>[3x]MATKGTKRSYEQMETDGERQNATEIRASVGKMIDGIGRFYIQMCTELKLSDYEGRLIQNSLTIERMVLSAFDERRNKYLEEHPSAGKDPKKTGGPIYRRVDGKWRRELILYDKEEIRRIWRQANNGDDATAGLTHMMIWHSNLNDATYQRTRALVRTGMDPRMCSLMQGSTLPRRSGAAGAAVKGVGTMVMELIRMIKRGINDRNFWRGENGRRTRIAYERMCNILKGKFQTAAQRTMVDQVRESRNPGNAEFEDLIFLARSALILRGSVAHKSCLPACVYGSAVASGYDFEREGYSLVGIDPFRLLQNSQVYSLIRPNENPAHKSQLVWMACHSAAFEDLRVSSFIRGTKVVPRGKLSTRGVQIASNENMETMESSTLELRSRYWAIRTRSGGNTNQQRASSGQISIQPTFSVQRNLPFDRPTIMAAFTGNTEGRTSDMRTEIIRLMESARPEDVSFQGRGVFELSDEKATSPIVPSFDMSNEGSYFFGDNAEEYDN

Following increased insights into the importance of vRNPs, antiviral drugs that target nucleoprotein (NP) are an attractive strategy as NP is a highly conserved multifunctional protein that plays an essential role in infection by all subtypes of IAVs during the virus infection life cycle. NP was reported to interact with RNA and oligomerize by self-interaction to form an oligomer to maintain the structure of RNP. In addition, NP is essential for viral transcription and replication; the major role of NP is the encapsidation of RNA into an RNP complex and maintenance of the conformation of the RNA template in a suitable order for transcription, replication, and assembly into virions. Furthermore, NP or RNPs participate in translocation between the cytoplasm and nucleus with the help of other viral proteins and host factors.

Here, we characterized a novel influenza A virus nucleoprotein (NP) inhibitor, FA-6005, that inhibited a broad spectrum of human pandemic and seasonal influenza A and B viruses in vitro and protects mice against lethal influenza A virus challenge. To obtain structural insights into the interaction between NP and FA-6005, FA-6005 was cocrystallized with NP, and the complex structure was determined. The NP/FA-6005 complex crystal belongs to space group C2221, with only one NP trimer in each asymmetric unit. Three FA-6005 molecules were found in each trimer. One was in the I41 pocket, and the major interactions involved in the I41 pocket included (i) hydrophobic interactions of the t-butyl group with G288, V285, and A286, ring C with I41, and ring D with G54 and R55; (ii) hydrogen bonding between amide O2 and T45; and (iii) dipole-dipole interactions of ring D with D51 and S283. The second one was in the Y289 pocket, and the interactions involved in the Y289 pocket included hydrophobic interactions of the t-butyl group and ring A with Y289, R305, and L306 and rings A and B with N309. The third one was around N224. However, N224 might not be a real pocket since the compound is seated between two symmetry-related NP molecules. We found that in the presence of FA-6005, mutation of residues in the I41 pocket displayed high resistance, while that of residues in the Y289 pocket exhibited more tolerance to the compound. FA-6005 would bind on the external surface of the NP, and thus, it may not interfere with the interaction between NPs during oligomerization.>GSMEGPAGYLRRADVAQLTQELGTAFFQQQQLPAAMADTFLEHLCLLDIDSEPVAARSTSIIATIGPASRSVERLKEMIKAGMNIARLNFSHGSHEYHAESIANVREAVESFAGSPLSYRPVAIALDTKGPGSGPGLSEQDVRDLRFGVEHGVDIVFASFVRKASDVAAVRAALGPEGHGIKIISKIENHEGVKRFDEILEVSDGIMVARGDLGIEIPAEKVFLAQKMMIGRCNLAGKPVVCATQMLESMITKPRPTRAETSDVANAVLDGADCIMLSGETAKGNFPVEAVKMQHAIAREAEAAVYHRQLFEELRRAAPLSRDPTEVTAIGAVEAAFKCCAAAIIVLTTTGRSAQLLSRYRPRAAVIA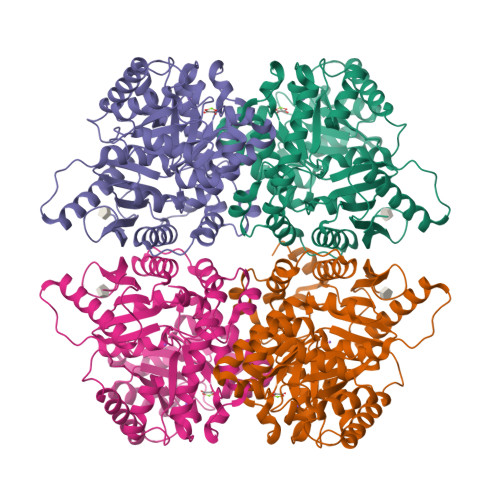VTRSAQAARQVHLCRGVFPLLYREPPEAIWADDVDRRVQFGIESGKLRGFLRVGDLVIVVTGWRPGSGYTNIMRVLSIS[8x]> MTTVTSYPGVYIEELNSLALSVSNSATAVPVFAVDEQNQYISEDNAIRINSWMDYLNLIGNFNNEDKLDVSVRAYFANGGGYCYLVKTTSLEKIIPTLDDVTLLVAAGEDIKTTVDVLCQPGKGLFAVFDGPETELTINGAEEAKQAYTATPFAAVYYPWLKADWANIDIPPSAVMAGVYASVDLSRGVWKAPANVAL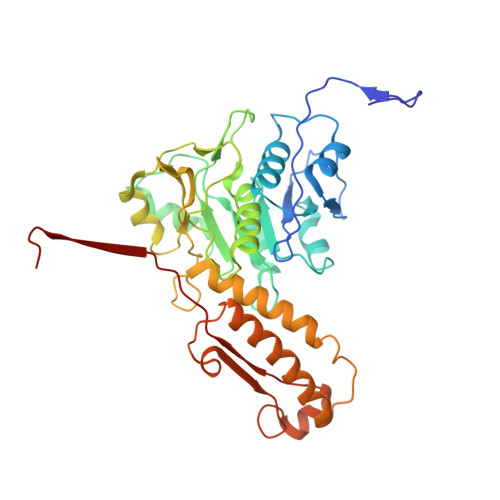KGGLEPKFLVTDELQGEYNTGRAINMIRNFSNTGTTVWGARTLEDKDNWRYVPVRRLFNSVERDIKRAMSFAMFEPNNQPTWERVRAAISNYLYSLWQQGGLAGSKEEDAYFVQIGKGITMTQEQIDAGQMIVKVGLAAVRPAEFIILQFTQDVEQR>GSGEEVSEEGFQIPATITERYKVGRTIGDGNFAVVKECVERSTAREYALKIIKKSKCRGKEHMIQNEVSILRRVKHPNIVLLIEEMDVPTELYLVMELVKGGDLFDAITSTNKYTERDASGMLYNLASAIKYLHSLNIVHRDIKPENLLVYEHQDGSKSLKLGDFGLATIVDGPLYTVCGTPTYVAPEIIAETGYGLKVDIWAAGVITYILLCGFPPFRGSGDDQEVLFDQILMGQVDFPSPYWDNVSDSAKELITMMLLVDVDQRFSAVQVLEHPWVNDDGLPENEHQLSVAGKIKKHFNTGPKPNSTAAGVSVIA[2x]

Doublecortin-like kinase 1 (DCLK1) is a multi-domain bi-functional protein that belongs to the protein kinase superfamily and the doublecortin (DCX) family within the microtubule-associated protein (MAP) superfamily. Doublecortin-like kinase 1 (DCLK1) is an understudied bi-functional kinase with a proven role in tumour growth and development. Multiple isoforms of DCLK1 exist, generated by alternative splicing. Here, we report the crystal structures of DCLK1 kinase domain in complex with DCLK1-IN-1 and its precursors.

Based on our initial structural information, two compounds were designed by Ferguson et al., introducing ethyl (FMF-03-055-1) and trifluoroethyl (DCLK1-IN-1) substituents at the R4 position 28 to improve selectivity towards DCLK1 by targeting the deep hydrophobic back pocket surrounded by residues Leu440, Val449, Met465 and the backbone of the DFG loop. To better understand how the ethyl substitution at position R4 provided increased potency towards DCLK1 and increased selectivity over ERK5, we solved the crystal structure of DCLK1-Cter:FMF-03-055-1 (residues 372-686) to 3.1 Å resolution. The backbone H-bond interactions mediated by Val468 located in the hinge region are still conserved in DCLK1-Cter:FMF-03-055-1. Our crystal structure reveals that the R4 ethyl group in FMF-03-055-1 indeed mediates additional contacts with Lys419, Ala417, Val404 and the gatekeeper residue Met465 as compared to the R4 methyl in XMD8-85. In addition to enhancing binding to DCLK1, the R4 ethyl substitution also decreased off-target binding to ERK5. This could be attributed to the presence in ERK5 of a leucine instead of methionine as the gatekeeper residue (Leu137). The structures of DCLK1-KD in complex with the benzopyrimido-diazipinone scaffold analogues XMD8-85 and FMF-03-055-1 show a conventional type I binding mode and in both cases the glycine loop collapses allowing extensive interactions with ring B and ring D contributing to their affinity towards DCLK1. The key positioning of the methyl group in XMD8-85 and the ethyl group in FMF-03-055-1 at position R4 towards the gatekeeper residue, which controls the access to the back pocket within the ATP binding site, along with the difference in the nature of the gatekeeper residue between DCLK1 (Met465) and ERK5 (Leu137) have highlighted how selectivity for DCLK1 over ERK5  can be achieved. Binding of both XMD8-85 and FMF-03-055-1 stabilised by vdw interactions between ring A and Gly532 that precedes the DFG motif. It is likely that these interactions are contributing to the stabilisation of the activation loop in an active conformation with both the DFG motif and the αC helix adopting a typical active-in conformation stabilised by the canonical salt bridge interaction between β3 strand lysine (Lys419) and the αC helix glutamate (Glu436).>MEPLDELDLLLLEEDGGAEAVPRVELLRKKADALFPETVLSRGVDNRYLVLAVETSQNERGAEEKRLHVTASQDREHEVLCILRNGWSSVPVEPGDIVHLEGDCTSEPWIIDDDFGYFILYPDMMISGTSVASSIRCLRRAVLSETFRGSDPATRQMLIGTILHEVFQKAISESFAPERLQELALQTLREVRHLKEMYRLNLSQDEILCEVEEYLPSFSKWAEDFMRKGPSSEFPQMQLSLPSDGSNRSSPCNIEVVKSLDIEESIWSPRFGLKGKIAVTV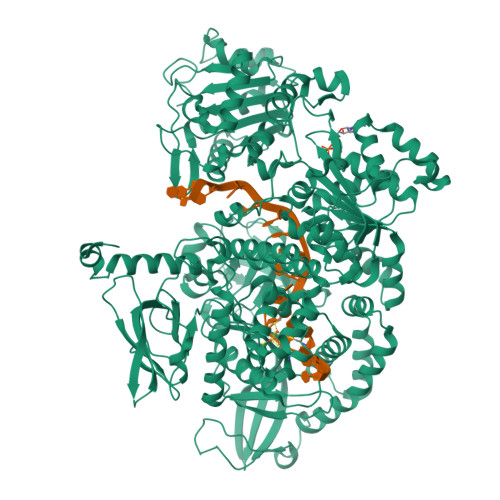GVKIHRDCKMKYKVMPLELKTGKESNSIEHRSQVVLYTLLSQERREDPEAGWLLYLKTGQMYPVPANHLDKRELLKLRNWLAASLLHRVSRAAPGEEARLSALPQIIEEEKTCKYCSQIGNCALYSRAVEEQGDDASIPEAMLSKIQEETRHLQLAHLKYFSLWCLMLTLESQSKDNRKTHQSIWLTPASELEESGNCVGNLVRTEPVSRVCDGQYLHNFQRKNGPMPATNLMAGDRIILSGEERKLFALSKGYVKKMNKAAVTCLLDRNLSTLPATTVFRLDREERHGDISTPLGNLSKLMESTDPSKRLRELIIDFREPQFIAYLSSVLPHDAKDTVANILKGLNKPQRQAMKRVLLSKDYTLIVGMPGTGKTTTICALVRILSACGFSVLLTSYTHSAVDNILLKLAKFKVGFLRLGQSHKVHPDIQKFTEEEICRSRSIASLAHLEELYNSHPIVATTCMGINHPIFSRKTFDFCIVDEASQISQPVCLGPLFFSRRFVLVGDHQQLPPLVVNREARALGMSESLFKRLERNESAVVQLTVQYRMNRKIMSLSNKLTYAGKLECGSDRVANAVLALPNLKDARLSLQLYADYSDSPWLAGVLEPDNPVCFLNTDKVPAPEQVENGGVSNVTEARLIVFLTSTFIKAGCSPSDIGVIAPYRQQLRIISDLLARSSVGMVEVNTVDKYQGRDKSLILVSFVRSNEDGTLGELLKDWRRLNVALTRAKHKLILLGSVSSLKRFPPLGTLFDHLNAEQLILDLPSREHESLSHIL[2x]> MAATTVNGGTVHFKGEVVNAACAVDAGSVDQTVQLGQVRTASLAQEGATSSAVGFNIQLNDCDTNVASKAAVAFLGTAIDAGHTNVLALQSSAAGSATNVGVQILDRTGAALTLDGATFSSETTLNNGTNTI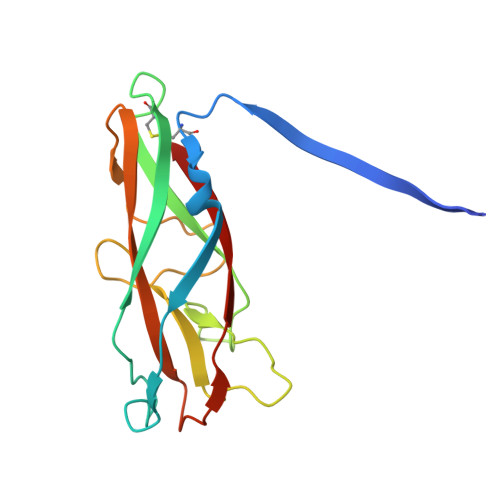PFQARYFATGAATPGAANADATFKVQYQ>MVMSYFDNFIKANQAYVDLHGTAHLPLKPK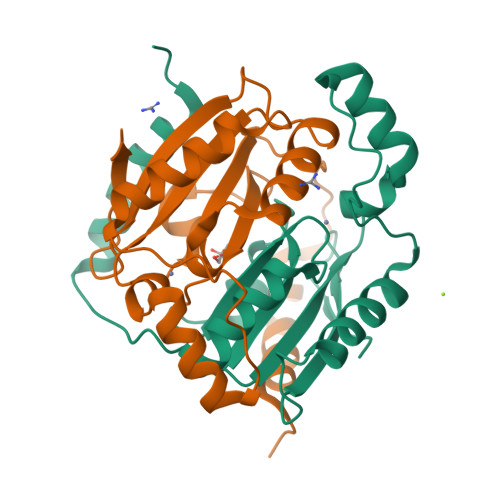TRVAIVTCMDSRLHVAPALGLALGDAHILRNAGGRVTDDVIRSLVISEQQLGTSEIVVLHHTDCGAQTFTNAEFTEQLKRDLAVDAGDQDFLPFTDIEESVREDIALLKNSPLIPEDIIISGAIYDVDTGRVREVN[2x]>MGSDKIHHHHHHENLYFQGMKKLNTNKLTEEQVNLFKNNLVYLATVDADGNPQVGPKGSMTVLDPSHLQYLEKTKGEAYENIKRGSKVALVAADVPSHTAVRVLATAEVHEDDDYAKKVLAKTEFPNAFVVNLNIEEV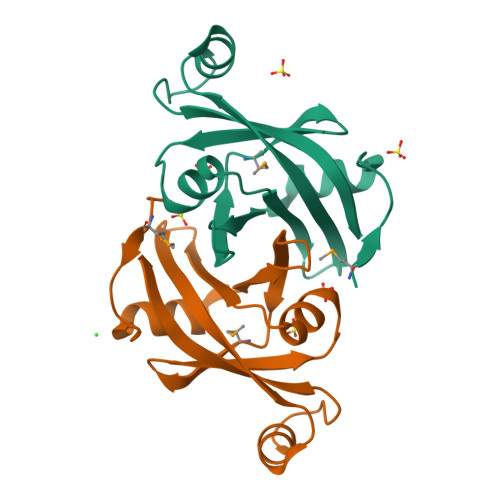FA[2x]> SSLK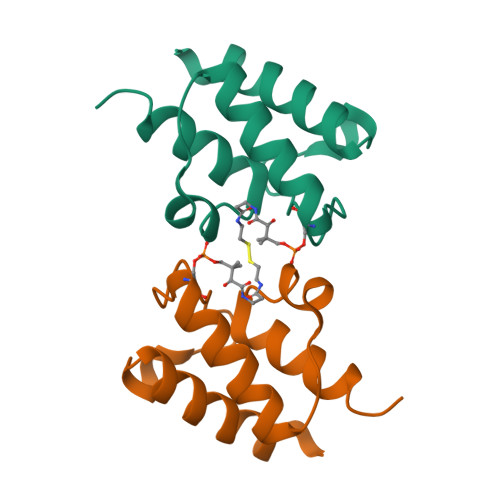STFDDIKKIISKQLSVEEDKIQMNSNFTKDLGADSLDLVELIMALEEKFNVTISDQDALKINTVQDAIDYIEKNNKQ> MSV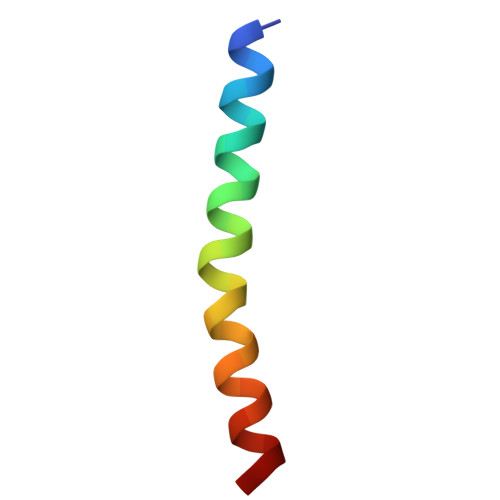LVYSFASFVLGWCLRSGITYFTRLMETSS>[2x]MDVEAFYKISYGLYIVTSESNGRKCGQIANTVFQLTSKPVQIAVCLNKENDTHNAVKESGAFGVSVLELET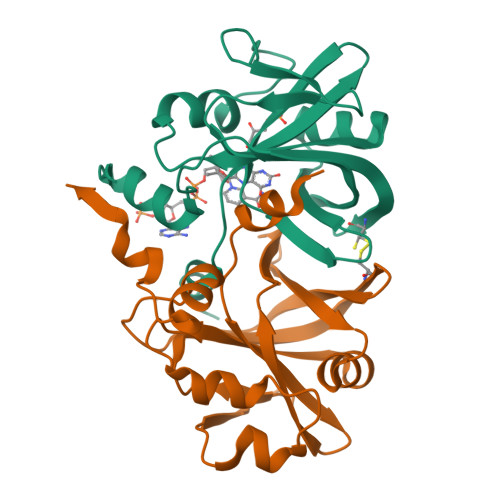PMEFIGRFGFRKSSEFEKFDGVEYKTGKTGVPLVTQHAVAVIEAKVVKECDVGTHTLFVGEAVDAEVLKDAEVLTYADYHLMKKGKTPRTATVYFESK>AVNFEVKDQTLMMELVPERLRGETATFDIEADGKVYVEKGRRVTARHIRQLEKDGVNFIEVPVEYIVGKVSAKDYVNEATGELIITANQEISLEALANLSQAG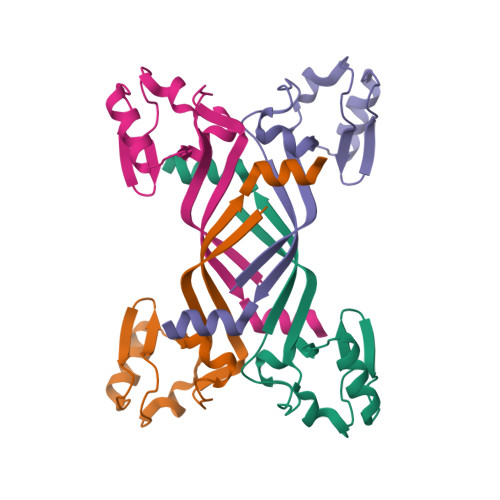[2x]> HDDHDHDHAHGSLGKHEHGVAQLNVALDGKTLELELDSPAMNLVGFEHAASTDADKAAVAKARAQLEKPLELFALPVTAGCSVASQELRSPLFGDKAPAHAHKEKAGHEHEHEHEHEHGHADIHAHYQLSCEKPELLKLLTLAEFF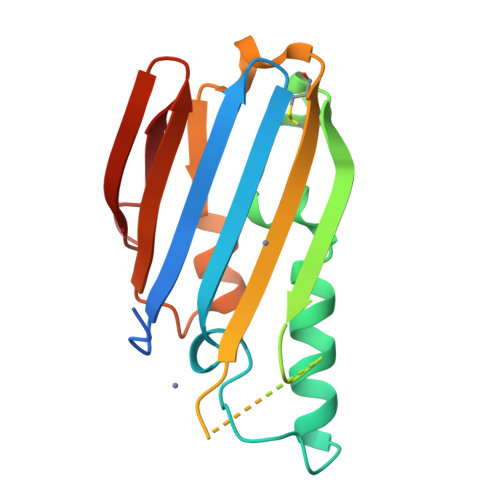KRFPATQKIQVQLIGPDGQKGADLAPASAELKL> MRGSHHHHHHTDPQGDAAQKTDTSHHDQDHPTFNKITPNLAEFAFSLYRQLAHQSNSTNIFFSPVSIATAFAMLSLGTKADTHDEILEGLNFNLTEIPEAQIHEGFQELLRTLNQPDSQLQLTTGNGLFLSEGLKLVDKFLEDVKKLYHSEAFTVNFGDTEEANKQINDYVEKGTQGKIVDLVKELDRDTVFALVNYIFFKGKWERPFEVKDTEEEDFHVDQVTTVKVPMMKRLGMFNIQHSKKLSSWVLLMKY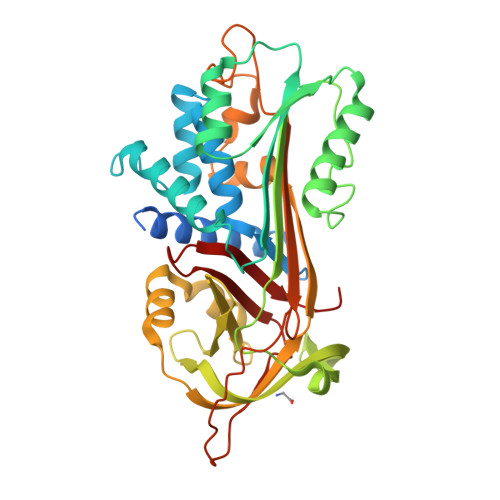LGNATAIFFLPDEGKLQHLENELTHDIITKFLENEDRRSASLHLPKLSITGTYDLKSVLGQLGITKVFSNGADLSGVTEEAPLKLSKAVHKAVLTIDEKGTEAAGAMFLEAIPMSIPPEVKFNKPFVFLMIEQNTKSPLFMGKVVNPTQK>GSNNSETPAPGPDSLLALAFPSDPQVSPDGKQVAFVLAQISEEDPAKPDKDFARPRYRSGLWLSEGGAARPLTHAETGRGDSAPRWSPDGQNLAFVRSAGEVKAALMLLPLKGGEARRVTHFKNGVSGPQWSPDGRFIAFTTTADTEDKRDERGEARVLTRPVYRANGADWLPERPAALWLYDVEADKLREWYAPEIGIGALSWWPD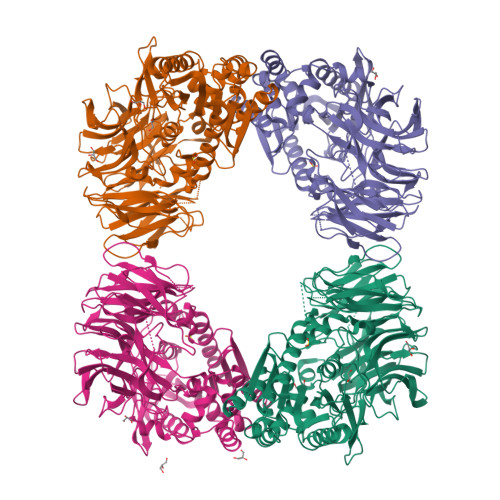SRGVLIVQSEDEWQASQWRQDVYDLPLPTADAPAAPQKLLDWNSAAHGLAPHPDGQRFALIGRPAGKGNTEHAHLYLIENGQHRRLDTGHDHPVGDAVGGDCHVGAFPEGPRWLDGDTLLFSSTVRGSVGLFTAHIGGGVKAYDHDPQGVISAFTANEHGVALIRESATRFPEVELNGQRVTDLHARFPFPVREPQRVTFETELGEGEGWVLLPEGEQKVPALLNIHGGPHTDYGHGFTHEFQLMAARGYGVCYSNPRGSVGYGQAWVDAIYGRWGTVDADDLLNFFDRCLEAVPRLDAAKTAVMGGSYGGFMTNWITGHTTRFQAAITDRCISNLISFGGTSDIGLRFWDDELGLDFSRRADALKLWDLSPLQYVENVKTPTLIVHSVLDHRCPVEQAEQWYAALHKHQVPVRFVRFPEENHELSRSGRPDRRLTRLNEYFAWLERWL[4x]> LGKFSQTCYNSAIQGSVLTSTCERTNGGYNTSSIDLNSVIENVDGSLKWQSPNFIETCRNTQLAGSSELAAECKTR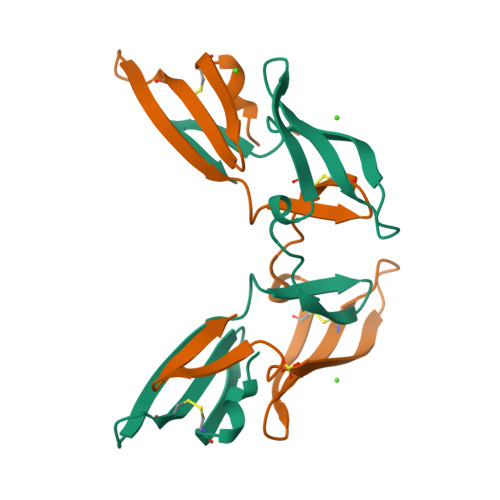AQQFVSTKINLDDHIANIDGTLKYE> MSIKPLHDRVVVKP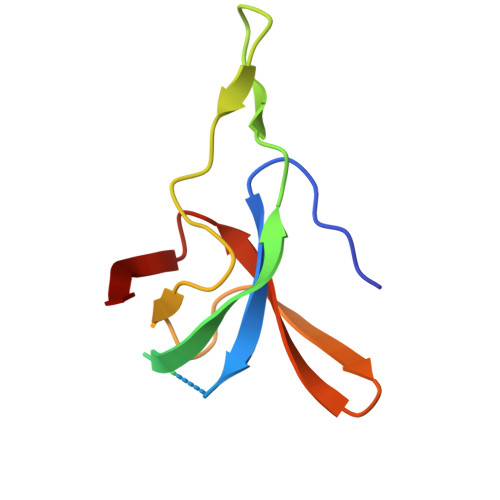IEADEVSAGGIVIPDSAKEKSTKGEVVAIGAGKPLDNGSLHAPVVKVGDKVIYGQYAGSSYKSEGVEYKVLREDDILAVIG UdgX excises uracil from uracil-containing DNA to concurrently form a covalent bond with the resulting AP-DNA. Structurally, UdgX is highly similar to family-4 UDGs (F4-UDGs). However, UdgX is unique in possessing a flexible R-loop (105KRRIH109). Our earlier studies allowed us to propose a reaction mechanism of UdgX, which involves the formation of a covalent bond between H109 of UdgX with the C1′ position of the target deoxyribose sugar concurrently with the uracil excision from this site in DNA.

Substitutions of His109 in MsmUdgX with Ser, Gly, Ala, Gln, Cys and Lys showed the loss of its covalent complex formation with DNA but gained canonical UDG activities. However, H109 substitutions by Gln or Lys, showed poor activity. However, to better understand the mechanism of uracil excision by the H109 mutants, we determined their structures along with a pentameric DNA, TTUTT by X-ray crystallography. The DNA backbone could not be modelled into the experimental electron density map in any of the mutant structures that were determined. Nonetheless, all structures revealed the excised uracil and the side chain substitutions at position 109. The structures also revealed invariant interactions of N91 and H178 with uracil. When we arranged the mutants in the order of increasing cavity sizes (left), we noted that the canonical UDG activity of the mutants increased with their increasing cavity sizes to begin with and then with a further increase in the cavity size, the UDG activity declined (right). It suggested that the initial increase in UDG activity (H109K to H109Q to H109G) occurred because of the efficiency with which the water molecule could be localized to make a nucleophilic attack on the C1′ position.

> AGAQDFVPHTADLAELAAAAGECRGCGLYRDATQAVFGAGGRSARIMMIGEQPGDKEDLAGLPFVGPAGRLLDRALEAADIDRDALYVTNAVKHFKFTRAAGGKRRIQKTPSRTEVVACRPWLIAEMTSVEPDVVVLLGATAAKALLGNDFRVTQHRGEVLHVDDVPGDPALVATVHPSSLLRGPKEERESAFAGLVDDLRVAADV In black-grass, upregulation of a phi (F)-class GST1 (AmGSTF1) has been shown to be a functional biomarker of MHR. Recombinant AmGSTF1 has been shown to exhibit both glutathione-S-transferase activity toward xenobiotics, as well as acting as a GPOX, reducing fatty-acid hydroperoxides to less reactive monohydroxy derivatives. The Phi (F) class GSTs, of which AmGSTF1 is an example, are found in all higher plants, being homodimeric enzymes in which each protomer of approximately 23–30 kDa with the catalytic serine residues located at the interface. Each protomer has two distinct domains; the N-terminal domain adopts the typical thioredoxin-fold, with the C-terminal domain being a bundle of at least five helices as demonstrated by the crystal structures of AmGSTF1 presented here.

To investigate the native AmGSTF1 active site in more detail, a cross-seeding approach was utilised whereby microseeds of the Phe122Thr variant crystals were used to obtain well-diffracting wild-type crystals in the tetragonal modification suitable for ligand soaking experiments. Following soaking with the glutathione-NBD conjugate, the crystals were found to diffract to 2.3 Å (Table S1b‡). The NBD-GS molecule was seen to bind across both the G and H sites, with the GSH portion of the molecule adopting the same conformation as the unconjugated GSH molecule seen in previous structures and the NBD moiety extending into the upper portion of the H-site. The aromatic portion of the molecule is seen to form a strong π-stacking interaction with Phe36, with its side-chain clearly rotated from its location in the apo-structure. The hydrophobic side chains of Phe122 and Met126 complete a narrow hydrophobic channel perfectly suited to bind the NBD moiety. These hydrophobic interactions help explain how the GS-NBD adduct acts as a strong competitive inhibitor following the conjugation of NBD-Cl. Interestingly, the GS-NBD conjugate in AmGSTF1 is seen to occupy a similar position to that observed for the related inhibitor 6-(7-nitro-2,1,3-benzoxadiazol-4-ylthio)hexanol (NBDHEX) and its respective GSH conjugate, as determined in the active site of HsGSTP1.14,21,31 In both cases, the inhibitor ligands are seen to form interactions both with residues in the α4 helix and the loop over the G-site. In HsGSTP1, these ligands are thought to stabilise GSH binding in the active site by preventing its conjugation with natural substrate molecules and subsequent dissociation. It is likely that the NBD derivatives play similar roles in AmGSTF1. Crystal structures of wild-type AmGSTF1, together with two specifically designed variants that allowed the co-crystal structure determination with glutathione and a glutathione adduct of the AmGSTF1 inhibitor 4-chloro-7-nitro-benzofurazan (NBD-Cl) were obtained. These studies demonstrated that the inhibitory activity of NBD-Cl was associated with the occlusion of the active site and the impediment of substrate binding.

> MAPVKVFGPAMSTNVARVTLCLEEVGAEYEVVNIDFNTMEHKSPEHLARNPFGQIPAFQDGDLLLWESRAISKYVLRKYKTDEVDLLRESNLEEAAMVDVWTEVDAHTYNPALSPIVYQCLFNPMMRGLPTDEKVVAESLEKLKKVLEVYEARLSKHSYLAGDFVSFADLNHFPYTFYFMATPHAALFDSYPHVKAWWDRLMARPAVKKIAATMVPPKA> SWQTYVDEHLMCDIEGTGQHLASAAIFGTDGNVWAKSSSFPEFKPDEINAIIKEFSEPGALAPTGLFLAGAKYMVIQGEPGAVIRGKKGAGGICIKKTGQAMVF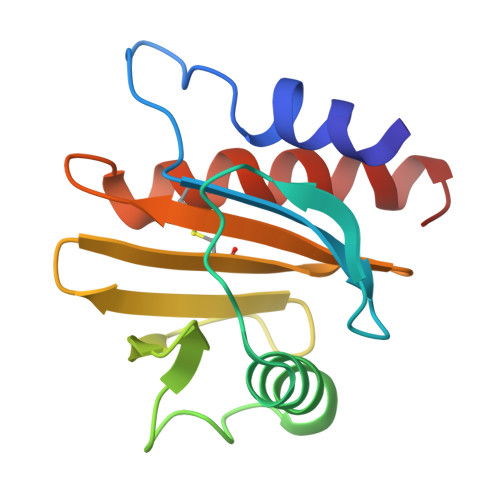GIYEEPVNPGQCNMVVERLGDYLVDQGM> TSSANEDMPVEKILEAELAVEPKTETYVEANMGLNPSSPNDPVTNICQAADKQLFTLVEWAKRIPHFSELPLDDQVILLRAGWNELLIASFSHRSIAVKDGILLATGLHVHRNSAHSAGVGAIFDRVLTELVSKMRDMQMDKTELGCLRAIVLFNPDSKGLSNPAEVEALREKVYASLEAYCKHKYPEQPGRFAKLLLRLPALRSIGLKCLEHLFFFKLIGDTPIDTFLMEMLEAPHQAT;> MSKESVRNDRNKKKKEVPKPECSESYTLTPEVGELIEKVRKAHQETFPALCQLGKYTTNNSSEQRVSLDIDLWDKFSELSTKCIIKTVEFAKQLPGFTTLTIADQITLLKAACLDILILRICTRYTPEQDTMTFSDGLTLNRTQMHNAGFGPLTDLVFAFANQLLPLEMDDAETGLLSAICLICGDRQDLEQPDRVDMLQEPLLEALKVYVRKRRPSRPHMFPKMLMKITDLRSISAKGAERVITLKMEIPGSMPPLIQEMLENSEGLD;> KHKILHRLLQDSS

The atRA isomer binds exclusively to RARs whereas the 9-cis form of RA binds to both RARs and RXRs, (each of which exists as three isoforms α, β and γ). A general model of RAR/RXR-mediated transcription proposes that unliganded RAR/RXR heterodimers are bound to regulatory elements of their target genes and interact with transcriptional repressor complexes such as NCOR/SMRT/SIN3 to recruit histone deacetylases that lead to repression of target gene transcription. Binding of agonist ligand to the nuclear receptor, triggers a conformational change in the ligand binding domain (LBD) with the repositioning of the C-terminal helix H12 creating a binding surface that allow coactivator to bind. As such, RAR/RXR is a non-permissive heterodimer in which RAR agonists can autonomously activate transcription while full responses to rexinoids occur only in the presence of RAR agonist ligands.

We now report the crystal structure of the heterodimer formed by the ligand binding domains of the human RARα bound to an agonist (all-trans retinoic acid, atRA) and the mouse RXRα bound to a rexinoid antagonist, LG100754 that has been shown to be an antagonist for RXR homodimer and a selective heterodimer antagonist. The crystal structure of the ternary molecular complex of RARα-atRA/RXRα-LG100754 LBDs and TIF-2 coactivator peptide was solved at 2.75 Å resolution and contains the two receptor LBDs bound to their respective ligands. One TIF-2 coactivator peptide is bound to RARα. The present structure adopts an asymmetric agonist/antagonist conformation. Indeed, RARα bound to atRA presents the active agonist conformation with the C-terminal helix H12 sealing the ligand binding cavity and one coactivator peptide bound through its LXXLL motif to the coactivator cleft generated by H3, H4 and H12. On the other side, the RXRα LBD bound to LG100754 adopts an antagonistic conformation with H12 pointing to the solvent and preventing the coactivator peptide from binding to RXR. The rexinoid antagonist LG100754 is buried in the LBP of RXRα formed by residues located on helices 3, 5, 7, 11 and the β-turn. The carboxylate group makes an anchoring salt bridge with Arg321 [hArg316] (H5) and hydrogen bond with amino group of Ala332 [hAla327] (LoopH5-H6) in the hydrophobic pocket, similarly as observed with the carboxylate of 9-cisRA in the RXRα complex. The propoxy group is pointing towards H11 and interacts with this helix through VDW contacts notably with Leu441 [hLeu436] which is repositioned. Indeed, the propoxy group of LG100754 induces a steric hindrance with Leu446 [hLeu441] in the LoopH11-H12 as observed in the RXR-oleic acid antagonist conformation, precluding H12 binding to the coactivator cleft.> MVLSDKELFAINKKAVEQGFNVKPRLNYNTVSGVNGPLVILEKVKFPRYNEIVNLTLPDGTVRQGQVLEIRGDRAIVQVFEGTSGIDVKKTTVEFTGESLRIPVSEDMLGRIFDGSGRPIDNGPKVFAEDYLDINGSPINPYARIYPEEMISTGVSAIDTMNSIARGQKIPIFSASGLPHNEIAAQICRQAGLVRPTKDVHDGHEENFSIVFAAMGVNLETARFFKQDFEENGSLERTSLFLNLANDPTIERIITPRLALTTAEYLAYQTERHVLTILT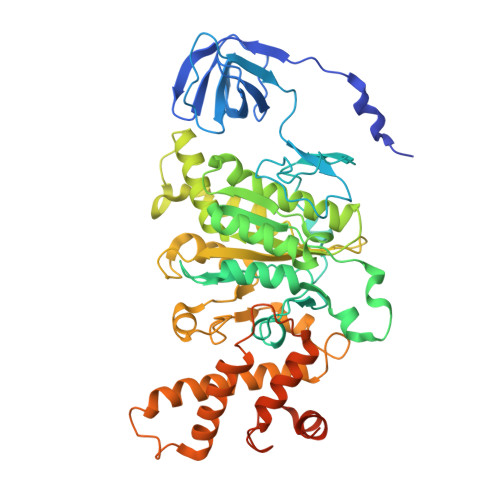DMSSYADALREVSAAREEVPGRRGYPGYMYTDLSTIYERAGRVEGRNGSITQIPILTMPNDDITHPIPDLTGYITEGQIFVDRQLHNKGIYPPINVLPSLSRLMKSAIGEGMTRKDHGDVSNQLYAKYAIGKDAAAMKAVVGEEALSIEDKLSLEFLEKFEKTFITQGAYEDRTVFESLDQAWSLLRIYPKEMLNRISPKILDEFYDRARDDADEDEEDPDTRSSGKKKDASQEESLI> GSHMVRKNPKSDKFKVKRFHHIEFWCGDATNVARRFSWGLGMRFSAKSDLSTGNMVHASYLLTSGDLRFLFTAPYSPSLSAGEIKPTTTASIPSFDHGSCRSFFSSHGLGVRAVAIEVEDAESAFSISVANGAIPSSPPIVLNEAVTIAEVKLYGDVVLRYVSYKAEDTEKSEFLPGFERVEDASSFPLDYGIRRLDHAVGNVPELGPALTYVAGFTGFHQFAEFTADDVGTAESGLNSAVLASNDEMVLLPINEPVHGTKRKSQIQTYLEHNEGAGLQHLALMSEDIFRTLREMRKRSSIGGFDFMPSPPPTYYQNLKKRVGDVLSDDQIKECEELGILVDRDDQGTLLQI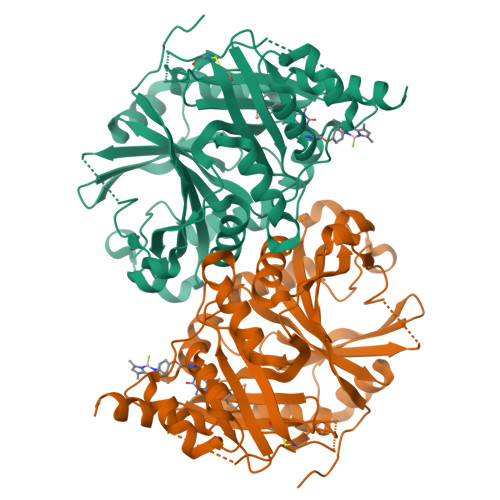FTKPLGDRPTIFIEIIQRVGCMMKDEEGKAYQSGGCGGFGKGNFSELFKSIEEYEKTLEAKQLVG>SDDRFLREKQAKLAEKIREFNDARQRGTPFYICRDLADLESKSGDRHGPHIVEAYRAVMEMVGEHPDAGEAPRERQFAKMYLDPNTQSANALAMRKQILKGATTFLEKQFWNEVNSLIAKYPQDANLGGLPDVVSKIKAYIRLRIARKTLVPDNVELQQINGEYVWAIVFYLLRAGFVTEAAQYVNSNQAHFRAIDRTFSGYINSYASSEERRLKRQMQDRCMSEYNQRIRNAPEGSIDPFRMACYKIIGRCDLSNRSLDGLQTDVNDWIWLQFNLARETDRSLELAGESYGLAELQASIREIGLKHFPKTAAEDTNGSFGMFFYLQILAGMFEQAIAYLYPFSYVDAVHFAIALTYYGLLRPVDAASAGNELLSHNTRSMPQINFGRMLGYYTRDFRAANPAAAVDYLVLICLNADEAAGGQQAQAALCHEALRELVLESREFSRLIGDIRPDGRRIRGVIEERGPLIALGQEDDFIRTITLQAASFADDNGRTTDAVLLYHLAEDYDTVVSIVSRALSEAISLEIGEDPMRLIPVKPRVTNAEGQVEEAAPGSSLSLAAIDDPVELAKAMMGMYERDHMFWQKIREPNRVACSVLLQMADIKSLVEQGRWAECLDKIRALDILPLTARGDPGTIRSYAARFPSLAQPV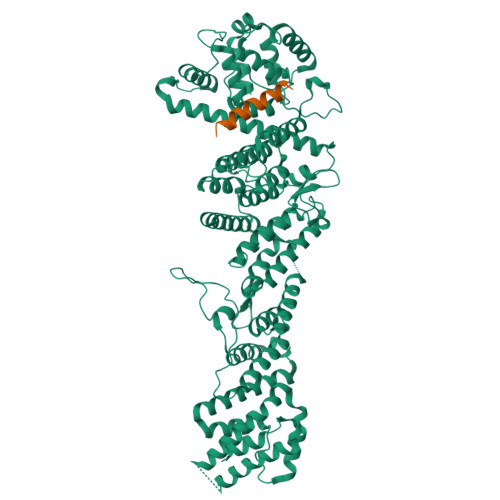AINVPNLLMWTVLCCMRQRERLAGGQFAGNESTARLMMDELKQMTVDLMAYTSQLRYRLPPHLHEALARASAD[2x];>[2x]SQQDGSLRSRKANLETGAFGKSTRRTRSKAATPAKREDPTIAAADKIFSNWLASQ>[4x]HAMVSNAETETEKEQEEAAAASEELPVMPWATSVASGYTLLRDPHHNKGLAFTEEERDGHYLRGLLPPAVLSQELQIKKFMNTLRQYQTPLQRYIAMMNLQETDERLFYKLLIDNVVELLPFVYTPTVGEACQKYGSIFRRPQGLYVSLKDKGKVLEVLRNWPHRNIQVICVTDGERILGLGDLGCQGMGIPVGKLALYTALGGVDPSVCLPITIDVGTNNEKLLNDEFYIGLRQKRATGEEYDELIEEFMSAVKQFYGEKVLIQ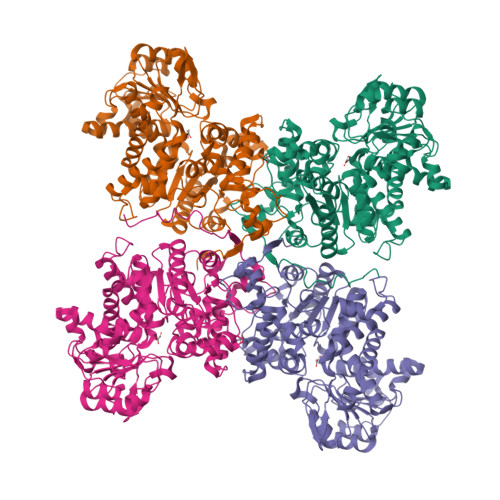FEDFANHNAFDLLEKYSKSHLVFNDDIQGTASVVLAGLLAALKMVGGTLAEQTYLFLGAGEAGTGIAELIALEISKQTNAPIEECRKKVWLVDSKGLIVDSRKGSLQPFKKPWAHEHEPLKTLYDAVQSIKPTVLIGTSGVGRTFTKEIIEAMSSFNERPIIFSLSNPTSHSECTAEQAYTWSQGRSIFASGSPFAPVEYEGKTFVPGQSNNAYIFPGLGLGLVISGAVRVHEDMLLAASKALADQATQDNFEKGSIFPPFTSIRKISAHIAAAVAAKAYELGLATRLPPPSDLVKYAENCMYTPVYRNYR A prototype of a Gram-negative epsilon/zeta TA module, the epsilon_1/zeta_1 (ngε_1/ngζ_1) TA system, is encoded by Neisseria gonorrhoeae, an obligate human pathogen causing the sexually transmitted disease gonorrhoea. Thereby, we identified a yet undescribed enzymatic activity. This proteobacterial zeta toxin phosphorylates UDP-activated sugar species at the C4′-OH group of the hexose moiety which eventually causes a lytic phenotype. The toxic activity is inhibited by co-expression of ngε_1 antitoxin, corroborating that the ngε_1 / ngζ_1 locus encodes for a toxin/antitoxin pair. As expected for a bona-fide type II TA system, we demonstrated protein-protein complex formation between ngε_1 and ngζ_1, which assemble into a heterodimeric complex.

Since we found UNAM to be a superb substrate in vitro compared to all other candidates which we identified by small metabolite extracts, we soaked UNAM into crystals and determined the structure of the complex. Indeed we observed a strong electron density for a UNAM molecule positioned in the active site of all four ngζ_1 polypeptide chains. To our surprise, Asp56, which most likely deprotonates the substrate before nucleophilic attack on the γ-phosphate group, is in hydrogen bonding distance to the C4′-OH group of the hexose moiety of UNAM, substantiating phosphorylation of this particular group. We observed a number of interactions between ngζ_1 and UNAM and nearly all residues that form hydrogen bonds with UNAM are strictly conserved among homologues, but not in authentic UNAG-3′ kinases. Most importantly, Asn75 and Lys59 form hydrogen bonds with the 1-carboxyethyl group of UNAM which could explain the preference of UNAM over UNAG by ngζ_1. Moreover, Arg181 and Arg175 form a positively charged patch in the active site counteracting the negatively charged phosphate groups. As expected from our initial, qualitative in vitro characterization, these measurements confirmed the apparent KM for UNAM to be more than 10-fold smaller than for UNAG or UDP-glucose. While this value is rather similar for UNAG and UDP-glucose, it is increased by a factor of approximately 1000 for UNAM, suggesting that UNAM-4P should be the predominant phosphorylated species also in vivo.

>MNKVEPQESNAIRMIKEACEKNRRMMTDEAFRKEVEKRLYAGPSPELLAKLRVLWAANKEQ[4x];>MVKLSSDINLRDFGNNEYLSSVQDEAIRFATEQTDEILSLYSQHADTEGGRYVCADTFKELFPAFENKEDRATVNNAIHNSAAVLSSTQFDEVLKRDEPQKKEVIFVTGIPGSGKTSTVKNMMMQDTTKLLFEGQLARPQSAFRKIEQCLERNLEVTIVAVSMRAERASDNTYKRFNEYGRGASIGIMADIQANLPDGLKQIRDKFGDAVKIVGINQDRNSEFIDKFDDVIKMLSLGSQEQILGRLAEKIQSDFDSGKISRECFNQAKGSMDLESVFAKKEYSQQRVVTNSKGVTLETKSANELWSKVEQIPVTGMKAGIYLLGQAKKAETGQTYSGEIIYKDAAAVFQKTKNGLVRHNATHNEERLAKLVEIGQNVSIGSNKGKLIVKSLEYSAKKSISR[4x]> NKITPNLAEFAFSLYRQLAHQSNSTNIFFSPVSIATAFAMLSLGTKADTHDEILEGLNFNLTEIPEAQIHEGFQELLRTLNQPDSQLQLTTGNGLFLSEGLKLVDKFLEDVKKLYHSEAFTVNFGDTEEAKKQINDYVEKGTQGKIVDLVKELDRDTVFALVNYIFFKGKWERPFEVKDTEEEDFHVDQVTTVKVPMMKRLGMFNIQHCKKLSSWVLLMKYLGNATAIFFLPDEGKLQHLENELTHDIIT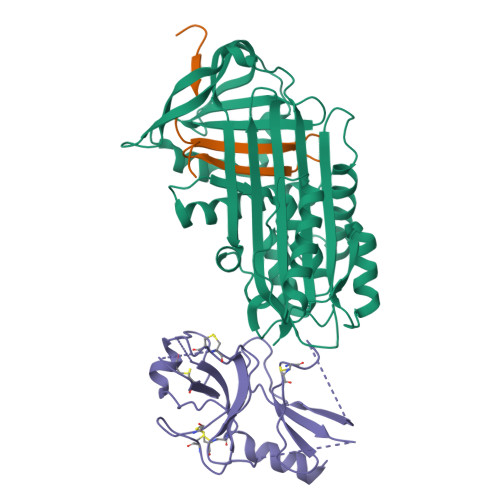KFLENEDRRSASLHLPKLSITGTYDLKSVLGQLGITKVFSNGADLSGVTEEAPLKLSKAVHKAVLTIDEKGTEAAGAMFLEAIPM;> SIPPEVKFNKPFVFLMIEQNTKSPLFMGKVVNPTQK;> FIFLALLGAAVAFPVDDDDKIVGGYTCGANTVPYQVSLNSGYHFCGGSLINSQWVVSAAHCYKSGIQVRLGEDNINVVEGNEQFISASKSIVHPSYNSNTLNNDIMLIKLKSAASLNSRVASISLPTSCASAGTQCLISGWGNTKSSGTSYPDVLKCLKAPILSDSSCKSAYPGQITSNMFCAGYLEGGKDSCQGDSGGPVVCSGKLQGIVSWGSGCAQKNKPGVYTKVCNYVSWIKQTIASN>[4x]MRGSHHHHHHGSQKTSDLIVLGLPWKTTEQDLKEYFSTFGEVLMVQVKKDLKTGHSKGFGFVRFTEYETQVKVMSQRHMIGGRWCDCKLPNSKQSQDEPLRSR

One example is TDP-43, which binds RNA and DNA and functions in mRNA splicing, translation regulation and transport1. However, when misfolded, TDP-43 aggregates and forms the major component in the ubiquitylated inclusions in the neuronal cells of patients with amyotrophic lateral sclerosis (ALS) and frontotemporal lobar degeneration (FTLD). TDP-43 consists of an N-terminal domain (NTD) and two tandem RNA recognition motifs, RRM1 and RRM2, followed by a C-terminal glycine-rich region (G). It forms homodimers and the two RNA-recognition motifs are involved in nucleic acid binding.

For the RRM1-D169G/DNA complex, the final refined model contained four RRM1 polypeptide chains (chain A to D) and four single-stranded DNA per asymmetric unit. The overall structure of RRM1-D169G mutant is similar to that of wild-type RRM1, nevertheless, a small local difference was observed in the β turn (Turn6) containing the D169G mutation. However in the D169G mutant, the β turn (Turn6) connecting the β4 and β5 strands, which contains the D169G mutation, shifted slightly due to the loss of the hydrogen bond between D169 and T115. The largest shift in the β turn is located around the mutation site G169 (chain A) whose Cα atom was shifted by 0.8 Å as compared to that of D169 of wild-type RRM1 (chain A). The β turn in all the four RRM1-D169G structures in the asymmetric unit has a similar shift of 1.0 Å (G169, Cα atom) on average as compared to wild-type RRM1 (D169, Cα atom), suggesting that this shift is inherent for the D169G mutant. We found that the D169G mutation consistently enhanced thermal stability in all TDP-43 constructs examined, with a larger melting point increase of 7–8 °C for the smaller RRM1 and N-RRM1 proteins and a smaller increase of 2–3 °C for the larger N-RRM12 and N-RRM12-G proteins. The crystal structure and MD simulations further reveal that the higher stability of D169G compared to wild-type TDP-43 is due to a local conformational change in the β turn region containing the D169G mutation and a reinforcement of the hydrophobic interactions in the core of RRM1. Here, we provide biochemical, structural, simulation, and cellular data to show that compared to wild-type TDP-43, the ALS-linked D169G mutation in TDP-43 generates a more stable protein that is cleaved by caspase 3 more efficiently, producing increased levels of TDP-35, but not TDP-25. Since the stabilization effect resulting from the D169G mutation is more pronounced in smaller protein constructs such as RRM1 (+7.6 °C) than larger constructs such as N-RRM12 (+2.0 °C), the smaller TDP-35 could be stabilized more than the full-length TDP-43 by the D169G mutation and hence, the TDP-43 D169G mutant is more susceptible to caspase 3 digestion.> MTKNYYDRSVSPVEYAYFDQSQNMRAINWNKIVDEKDLEVWNRVTQNFWLPENIPVSNDLPSWNELDDDWQQLITRTFTGLTLLDTVQSSIGDVAQIKNSLTEQEQVIYANFAFMVGVHARSYGTIFSTLCTSEQIEEAHEWVVDNEALQARPKALIPFYTADDPLKSKIAAALMPGFLLYGGFYLPFYLSARGKLPNTSDIIRLILRDKVIHNFYSGYKYQLKVAKLSPEKQAEMKQFVFDLLDKMIGLEKTYLHQLYDGFGLADEAIRFSLYNAGKFLQNLG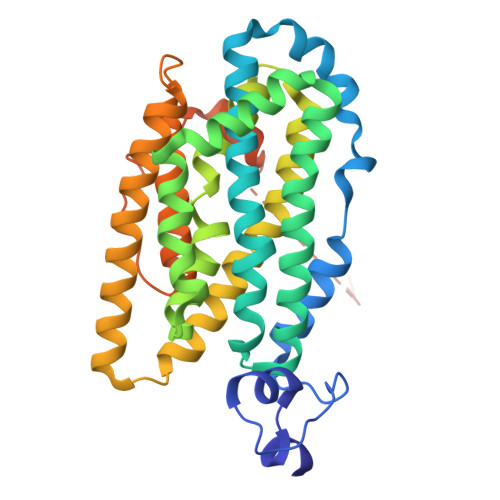YESPFTKEETRIAPEVFAQLSARADENHDFFSGSGSSYIIGTSEETLDEDWDF(13E,15S)-15-hydroxy-9-oxoprosta-10,13-dien-1-oic acid | C20 H32 O4 | 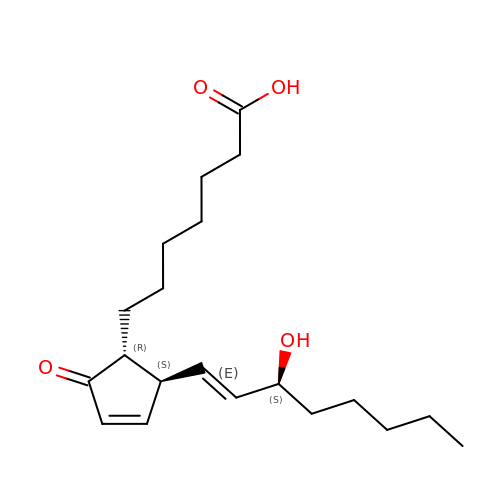BGKHCLZFGPIKKU-LDDQNKHRSA-N>[2x]MNIRLHGLTTILSALVVLTAPTAVLAQDNLVTGELITTVNSGTPGKGGEVTFAVTRDITNWNVTSALGNNAVVRTVTLPIVPSAFMVQPDFTLKMNTDLLESAELTSTDPQTVVYRIREDAVWSDGVPITGDDFIYFWKTQNRRDCPECLINASYGHDFIETLEQDETGKVVTATFSEPFLGWQGLFMFLYPAHLAEKHGDIAESYNNFLSNEVPAWSGGPYMVESFDPGQLVTLVPNP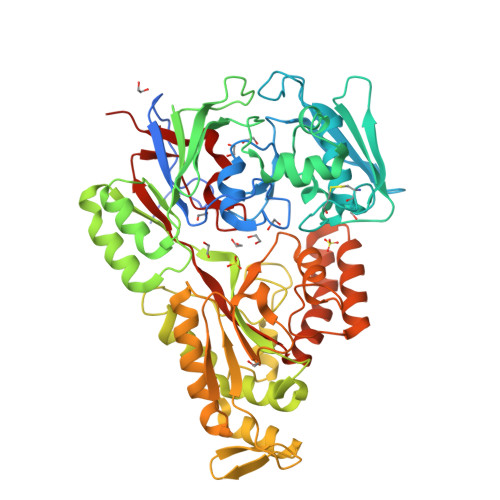KWYGEKGPYLDKLKFRIITDSTQQLTALENGEVDVIYPQGATQDMVEQAAGLDYLGIDFQMNPSANWYFMGLNSKAGPMSDIALRKAVLTAIDAGDLKAKTADPYLRNWPHMGSVMFLPNQAGYADRRGARGYGTGDVEKAKGILSEAGYKLSGGSLLDPSGKPVSTLRLSFPPGYPAANDMARLITGYIAPLGLKTDLLTGPNATADYLLSGNFDLHLNYFSQQVFPAVKAGQIFLRDTRQNYFGFNDPKIEEIIGKAAAASSIEESAAILSEADELAMDYAALFPIYQLPTALIYKEAILNLRDNPNQLGPAYNTAEWGLAELEHHHHHH> GEERGRILISLKYSSQKQGLLVGIVRCAHLAAMDANGYSDPYVKTYLKPDVDKKSKHKTAVKKKTLNPEFNEEFCYEI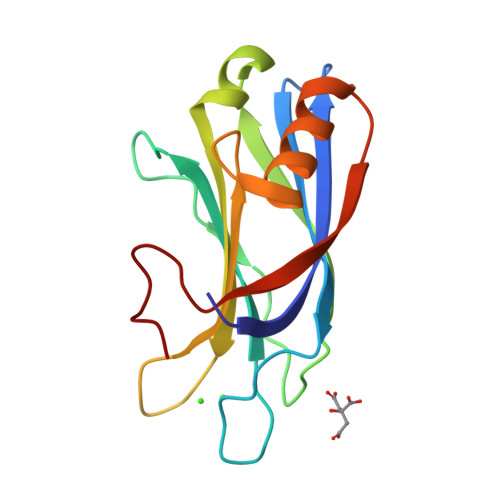KHGDLAKKTLEVTVWDYDIGKSNDFIGGVVLGINAKGERLKHWFDCLKNKDKRIERWHTLTNEIPGAVLSD> AAPGKPTIAWGNTKFAIVEVDQAATAYNNLVKVKNAADVSVSWNLWNGDTGTTAKVLLNGKEAWSGPSTGSSGTANFKVNKGGRYQMQVALCNADGCTASDATEIVVADTDGSHLAPLKEPLLEKNKPYKQNSGKVVGSYFVEWGVYGRNFTVDKIPAQNLTHLLYGFIPIC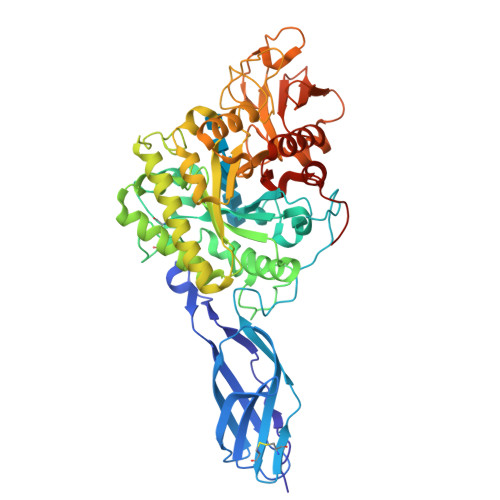GGNGINDSLKEIEGSFQALQRSCQGREDFKVSIHDPFAALQKAQKGVTAWDDPYKGNFGQLMALKQAHPDLKILPSIGGWTLSDPFFFMGDKVKRDRFVGSVKEFLQTWKFFDGVDIDWEFPGGKGANPNLGSPQDGETYVLLMKELRAMLDQLSVETGRKYELTSAISAGKDKIDKVAYNVAQNSMDHIFLMSFDFYGAFDLKNLGHQTALNAPAWKPDTAYTTVNGVNALLAQGVKPGKIVVGTAMYGRGWTGVNGYQNNIPFTGTATGPVKGTWENGIVDYRQIAGQFMSGEWQYTYDATAEAPYVFKPSTGDLITFDDARSVQAKGKYVLDKQLGGLFSWEIDADNGDILNSMNASLGNSAGVQ>[14x]MNPMYVSKLSLVLVAAALVGACATKPAPDFGGRWKHVNHFDEAPTEIPLYTSYTYQATPMDGTLKTMLERWAADSNMQLSYNLPSDYTLIGPVSAISTTSVQQAATELSAVYAAQGVSVSVSANKLLVQPVPVSSGAKL;>[14x]MKLFNRYRVALLSALPLALCALSAAAQVVQEYEYAPDRIYQVRTGLGITTQVELSPNEKILDYSTGFTGGWELTRRENVFYLKPKNVDVDTNMMIRTATHSYILELKVVATDWQRLEQAKQAGVQYKVVFTYPKDTSFNNVADADTSKNGPLLNAKILKDRRYYYDYDYATRTKKSWLIPSRVYDDGKFTYINMDLTRFPTGNFPAVFAREKEHAEDFLVNTTVEGNTLIVHGTYPFLVVRHGDNVVG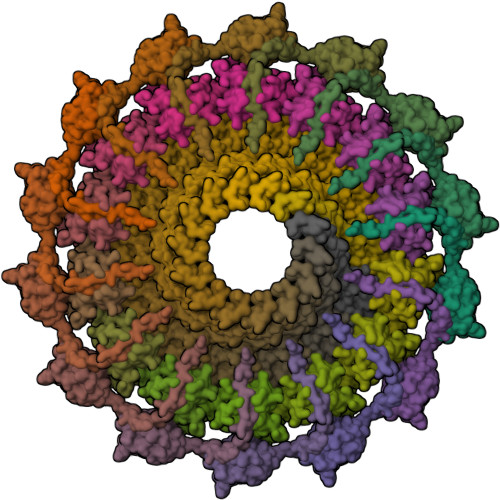LRRNKQK;>MNSNIPNSPDERIQNHGGDEQHNGDHNERNNPYFARQQASAEPDLDANEPILRSSDIKRLNRKALVFLAAIAALLILAIFWLATQSGEDSAPPKPRTETVVAPALPQSMTAPVEEAPVPLAQQPSLPPLPPMPTDNSEEVSSAPERQRGPTLLERRILAESAANGGGVPGQLGAQPAPTQEDGPVTLAKPISNPDGLLVRGTYIRCILETRIISDFGGYTSCIVTEPVYSINGHNLLLPKGSKMLGQYSAGEPTSHRLQVVWDRVTTPTGLDVTLMGPGIDTLGSSGHPGNYNAHWGNKIASALFISLLSDAFKYAAAEYGPETTTIGVGSGIVTQQPFESNTARSMQQLAEQAVEKSGRRPATLTINQGTVLNVYVAKDVDFSAVLPKAAALEGLSAWSHPQFEK[14x]>MATIQRIVRQASKLRVVFATDEEIAAHEARLDLVQKKGGSCLWRATRESGSIGSMSEPRFVHLRVHSDYSMIDGPAKTA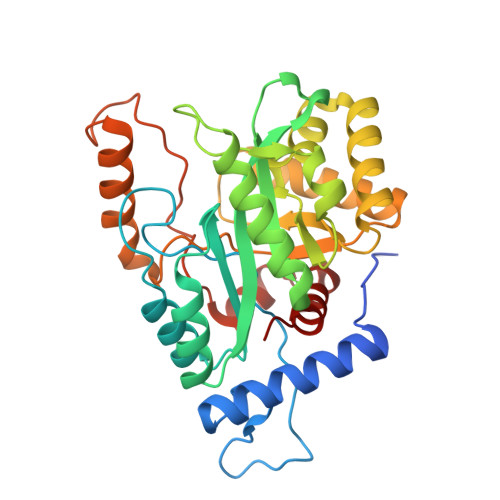PLVKKAAALGMPALAITDFTNLCGLVKFYGAGHGAGIKPIVGADFNVQCDLLGDELTHLTVLAANNTGYQNLTLLISKAYQRGYGAAGPIIDRDWLIELNEGLILLSGGRMGDVGRSLLRGNSALVDECVAFYEEHFPDRYFLELIRTGRPDEESYLHAAVELAEARGLPVVATNDVRFIDSSDFDAHEIRVAIHDGFTLDDPKRPRNYSPQQYMRSEEEMCELFADIPEALANTVEIAKRCNVT[4x]> SPQPLEQIKLSESQ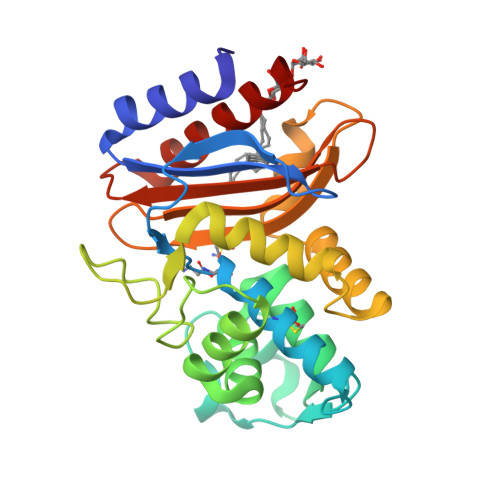LSGRVGMIEMDLASGRTLTAWRADERFPMMSTFKVVLCGAVLARVDAGDEQLERKIHYRQQDLVDYSPVSEKHLADGMTVGELCAAAITMSDNSAANLLLATVGGPAGLTAFLRQIGDNVTRLDRWATELNEALPGDARDTTTPASMAATLRKLLTSQRLSARSQRQLLQWMVDDRVAGPLIRSVLPAGWFIADKTGAGERGARGIVALLGPNNKAERIVVIYLRDTPASMAERNQQIAGIGAALIEHWQR[(3s,5s,7s)-adamantan-1-yl][4-(2-amino-5-chlorophenyl)piperazin-1-yl]methanone | C21 H28 Cl N3 O | 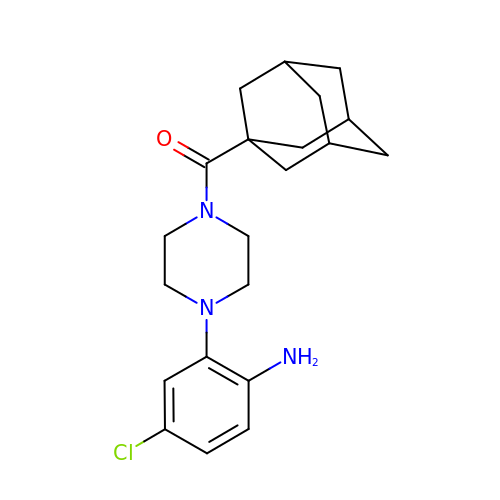SNWNZTLWPJKTEO-OFIQSVQDSA-N>[2x]MGRGKRRAKTRNIAIASTKEVQWQGIFMIIVWLCVMGSLIFFANPEASRRVFAKFSHLQSFYGATSVAFAFATGLDILAYVNAVSDEKRVLSGILAYVDGVACISYLSMATLNLYF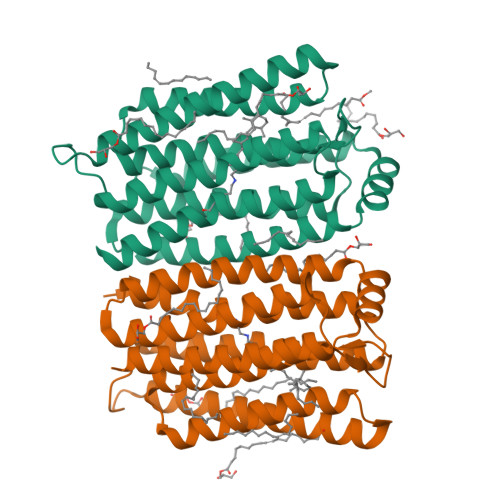LVDSTQGNPVWLMRYAEWIITCPTLLYWCGLASRADRSSVSDIATADALLLAGGALSSILPSWPAFFVFAGSFATYIYVMLHMWGMFGKAMQPDFQPPPPLPRHALHLLRCEIVMSWSIFPLVEFLRRQGYIDFQVGEAMNCVADYAAKVGLAMIMVNCNLEQINALRVENLYFQ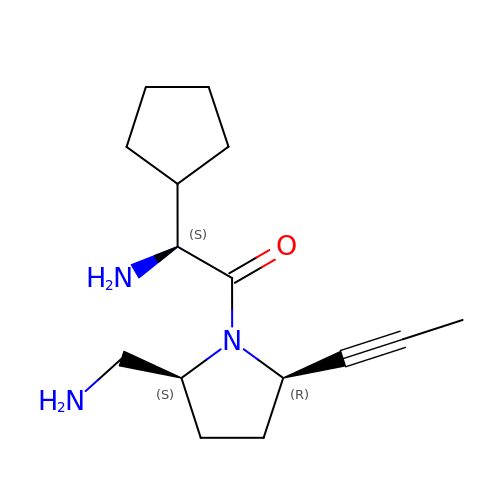(1S)-2-[(2S,5R)-2-(AMINOMETHYL)-5-PROP-1-YN-1-YLPYRROLIDIN-1-YL]-1-CYCLOPENTYL-2-OXOETHANAMINE | C15 H25 N3 O | RIKCMKYTGBHVSX-IHRRRGAJSA-N> MQDPNADTEWNDILRKKGILPPKESLKELEEEAEEE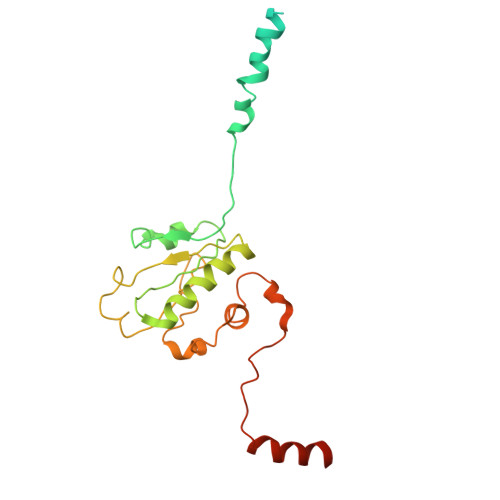QRILQQSVVKTYEDMTLEELEDHEDEFNEEDERAIEMYRRRRLAEWKATKLKNKFGEVLEISGKDYVQEVTKAGEGLWVILHLYKQGIPLCALINQHLSGLARKFPDVKFIKAISTTCIPNYPDRNLPTIFVYLEGDIKAQFIGPLVFGGMNLTRDELEWKLSESGAIMTDLEENPKKPIEDVLLSSVRRSVLMKRDSDSEGD>MSSSPVKRQRMESALDQLKQFTTVVADTGDFHAIDEYKPQDATTNPSLILAAAQMPAYQELVEEAIAYGRKLGGSQEDQIKNAIDKLFVLFGAEILKKIPGRVSTEVDARLSFDKDAMVARARRLIELYKEAGISKDRILIKLSSTWEGIQAGK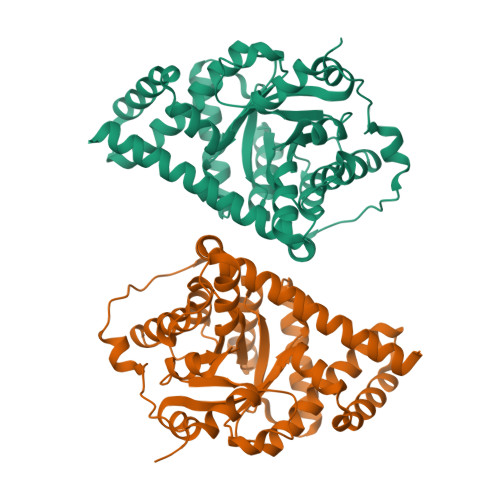ELEEQHGIHCNMTLLFSFAQAVACAEAGVTLISPFVGRILDWHVANTDKKSYEPLEDPGVKSVTKIYNYYKKFSYKTIVMGASFRNTGEIKALAGCDFLTISPKLLGELLQDNAKLVPVLSAKAAQASDLEKIHLDEKSFRWLHNEDQMAVEKLSDGIRKFAADAVKLERMLTERMFNAENGK[2x]>[3x]GGSEFMAGTALKRLMAEYKQLTLNPPEGIVAGPMNEENFFEWEALIMGPEDTCFEFGVFPAILSFPLDYPLSPPKMRFTCEMFHPNIYPDGRVCISILHAPGDDPMG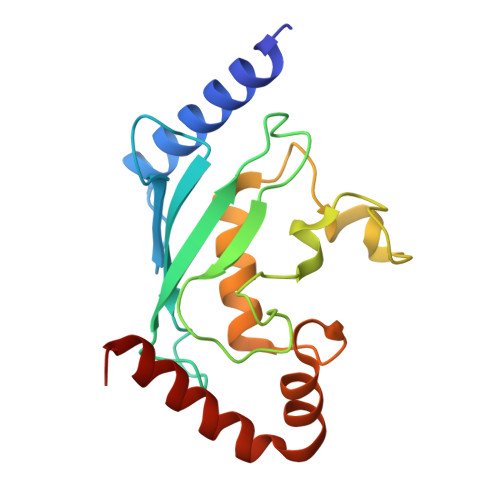YESSAERWSPVQSVEKILLSVVSMLAEPNDESGANVDASKMWRDDREQFYKIAKQIVQKSLGL>MAHHHHHHMDCQALAKSLEQMNHLHNVKYLEAKDLTDFNQKSAYYICHQIAEKQLSKEGGHVVIGLSGGKTPIDVYKNIALVKDIKIDTSKLIFFIIDERYKRDDHKFSNYNNIKFLFESLKINEKEQLYRPDTSKNIVECVRDYNEKIKNMVKKYTKVDIAILGMGSDFHIASLFPNIFFNIYMNNYQNSY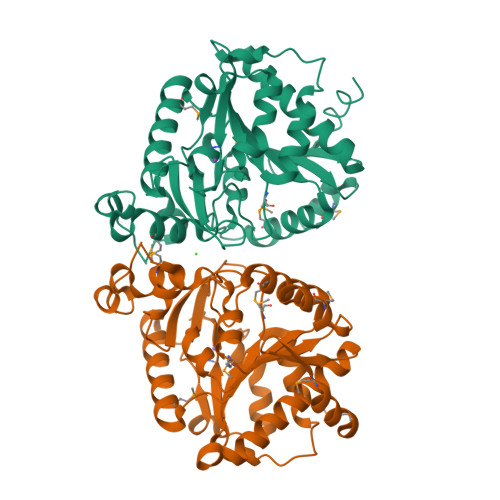IYDESSIKVANSNDTSDNDNLDLLKEYVYFTTTNNFDVRKRITVSLDLLGNASSKIFLLNSTDKLDLWKNMLLKSYVDVNYCLYPAVYLIDSMNTTVVTCGYTNYPQMLEDIYVSNSSLS[4x]Chromosomal replicative helicases are hexameric protein ensembles that travel ahead of the advancing replisome, dissolving duplex DNA into templates for DNA synthesis. Melting of the duplex arises from ATP dependent translocation of the helicase along single stranded (ss) DNA, paired with inclusion/exclusion of DNA strands from an internal chamber. To assemble such entities on DNA, bacteria use specialized loading factors that mediate opening of the protein ring, guiding of ssDNA into the exposed chamber, and, finally, sealing of the helicase with ssDNA trapped inside. E. coli DnaC serves as the helicase loader and delivers the DnaB helicase to the bacterial origin; it is unrelated in sequence to λP, the loader that operates at the λ phage origin, and which is the focus of this work.

We report on the structure of the Escherichia coli DnaB-helicase•bacteriophage λP helicase loader complex (henceforth: BP) by single particle cryoEM at 4.1 Å resolution. In the identified complex, we observe five λP loader molecules bound to the helicase at five consecutive DnaB subunit interfaces; the sixth DnaB interface has been breached, thus precluding a sixth λP from binding. The λP loader restructures layers in the DnaB helicase comprised of carboxy-terminal (CTD) and amino-terminal (NTD) domains into novel right-handed open spiral configurations. Restructuring breaks one of the six helicase subunit interfaces to produce ~15 Å and ~20 Å openings in the CTD and NTD layers, respectively; these openings are of sufficient size to enable access by ssDNA to the internal chamber of the DnaB-helicase. Furthermore, reconfiguration forces the CTD layer of the helicase into a restrained inactive conformation wherein the ATP hydrolytic and DNA-binding properties are diminished, if not abolished. Each λP protomer is comprised of a helical domain that binds in a deep gulley formed by an interface between two adjacent DnaB CTDs. Further, each λP protomer sends out a lasso-like segment that runs along the edge of the CTD and positions a λP helix against a site formed by the CTD and the linker helix (residues 183–194) of an adjacent DnaB subunit. Although our EM samples were prepared with a large excess of ATP, we observe that five of the six sites in the BP complex are occupied by ADP, while the sixth site, whose composite architecture involves subunits that span the breached CTD ring, lies unfilled. Taken together, our findings indicate that the λP helicase loader induces a conformation of the DnaB helicase that is neither optimal for DNA binding nor ATP hydrolysis. However, binding of the λP helicase loader is not compatible with the dilated form; indeed, the NTD and CTD tiers of the BP complex, by virtue of arrangement and size of internal chamber, are found in the constricted form.

>MAGNKPFNKQQAEPRERDPQVAGLKVPPHSIEAEQSVLGGLMLDNERWDDVAERVVADDFYTRPHRHIFTEMARLQESGSPIDLITLAESLERQGQLDSVGGFAYLAELSKNTPSAANISAYADIVRERAVVREMISVANEIAEAGFDPQGRTSEDLLDLAESRVFKIAESRANKDEGPKNIADVLDATVARIEQLFQQPHDGVTGVNTGYDDLNKKTAGLQPSDLIIVAARPSMGKTTFAMNLVENAAMLQDKPVLIFSLEMPSEQIMMRSLASLSRVDQTKIRTGQLDDEDWARISGTMGILLEKRNIYIDDSSGLTPTEVRSRARRIAREHGGIGLIMIDYLQLMRVPALSDNRTLEIAEISRSLKALAKELNVPVVALSQLNRSLEQRADKRPVNSDLRESGSIEQDADLIMFIYRDEVYHENSDLKGIAEIIIGKQRNGPIGTVRLTFNGQWSRFDNYAGPQYDDE[6x]>MSLRQLLSPVEFDPQQCDQTFTIATTDYAMQTILPFALPRIYQEAPNVSFNFLPLQHDRLSDQLTYEGADLAICRPTGPVEPLRSEILGRVGVLCLLSKQHPLANQEMSLDDYLSHPHAMIAISDGVKALIEQALIDKPQRKMVLRAYHLEAALAIVDTLPIIITVPADLAYLVAERYDLVVKPLPFQFTPFDY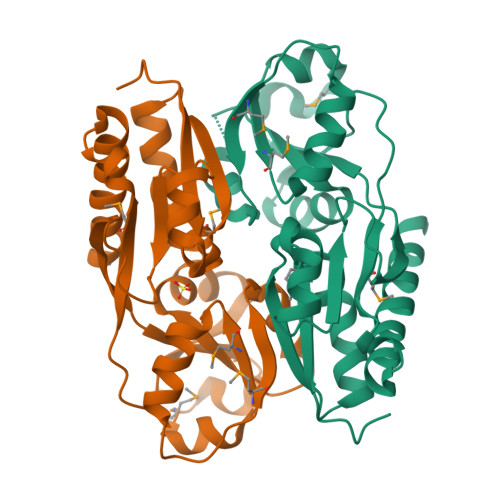SMIWHARCEHSPAQEWLRSVVREECSRLIAKRIEDMGLNEGHHHHHH[4x]> GSHMMEKIKVAIADDNKELVKTLESYLADHPQIEVITTAPNGK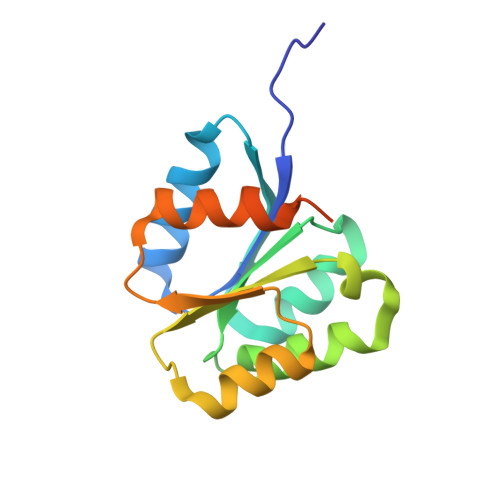VILSLMENDLPDVLLLDIIMPHLDGLAVLEMMQANENLSKVQVIMLTAFGQEDVMKQAVDLGASYFMLKPFEFDRLDNQILQVAGHKQEADQRSSILQSQPQPKT>[3x]SMVKEVVRTDSLKGRRGRLPSKPKSPQEPSPPSPPVSLISALVRAHVDSNPAMTS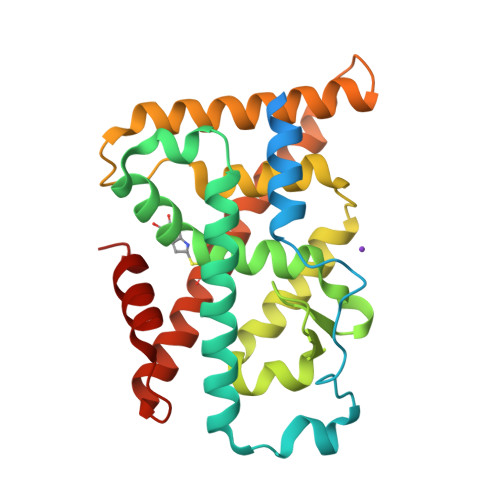LDYSRFQANPDYQMSGDDTQHIQQFYDLLTGSMEIIRGWAEKIPGFADLPKADQDLLFESAFLELFVLRLAYRSNPVEGKLIFCNGVVLHRLQCVRGFGEWIDSIVEFSSNLQNMNIDISAFSCIAALAMVTERHGLKEPKRVEELQNKIVNCLKDHVTFNNGGLNRPNYLSKLLGKLPELRTLCTQGLQRIFYLKLEDLVPPPAIIDKLFLDTLPF>M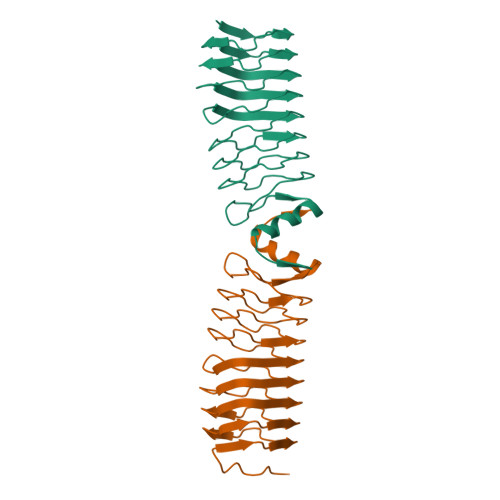PAKTLESKDYCGESFVSEDRSGQSLESIRFEDCTFRQCNFTEAELNRCKFRECEFVDCNLSLISIPQTSFMEVRFVDCKMLGVNWTSAQAGALSFERCILNDSLFYGLYLAGVKMVECRIHDANFTEADCEDADFTQSDLKGSTFHNTKLTGASFIDAVNYHIDIFHNDIKRARFSLPEAASLLNSLDIELSD[2x]> TQTQLAIDNVLASAESTIQLNELPKVVLDFITGEQTSVARSGGIFTKEDLINLKLYVRKGLSLPTRQDEVEAYLGYKKIDVAGLEPKDIKLLFDEIHNHALNWNDVEQAVLQQSLDLDIAAKNIISTGNEIINLINQMPITLRVKTLLGDITDKQLENITYESADHEVASALKDILDDMKGDINRHQTTTENVRKKVSDYRITLTGGELSSGDKVNGLEPQVKTKYDLMEKSNMRKSIKELDEKIKEKRQRIEQLKKDYDKFVGLSFTGAIGGIIAMAITGGIFGAKAENARKEKNALISEVAELESKVSSQRALQTALEALSLSFSDIGIRMVDAESALNHLDFMWLSVLNQITESQIQFAMINNALRLTSFVNKFQQVITPWQSVGDSARQLVDIFDEAIKEYKKVYG

We have unraveled structures of the soluble components and the pore assembly of the YaxAB cytolysin from Y. enterocolitica. The crystal structures show an atypical fold, comprising a head domain reminiscent of ClyA family toxins and pronounced coiled-coil and foot domains unique to the YaxAB system. In line with our finding that the isolated YaxA and YaxB head domains form spoked oligomers in solution, the YaxB head domain in isolation was sufficient for recruitment to membrane-bound YaxA. Together, our biochemical data support a role for YaxA as the initial membrane-interacting subunit of the toxin, able to bring the lytic effector YaxB to the target cell surface. Therefore, we propose that this class of toxins defines a new structural family of α-PFTs.

YaxA and PaxB crystal structures were determined using single-wavelength anomalous dispersion (SAD) on selenomethionine-derivatized proteins. Because our PaxB model could be well resolved, missing merely the N-terminal 11 residues, we will utilize these coordinates for most structural analyses throughout the manuscript. All three proteins adopt similarly elongated, α-helical folds composed of a five-helix bundle head domain and a two-helix-coiled-coil stalk, tapering to a narrow turn in the case of YaxA, while connecting to an additional α-helical domain in the case of PaxB. For alignments of the YaxA head domain, Z-scores ranged from 9.6 (soluble-monomeric ClyA, 5.5 Å RMSD; PDB code 1QOY34) to 12.2 (NheA, 3.4 Å RMSD; PDB code 4K1P26). Looking at a series of conserved and solvent-exposed hydrophobic residues of the YaxA foot domain, we suspected this moiety to be a possible membrane insertion site. Replacing individual nonpolar residues in the YaxA foot to aspartic acid (V264, L266, F268, and I272, along helix α4) resulted in 2-fold to 3-fold weaker membrane association (lanes 7–10). Strikingly, a deletion mutant of most of this domain (Δ265–284; Fig. 6c, lane 11) did not co-sediment with membranes. Reflecting their impaired membrane binding, YaxA foot domain mutants showed reduced hemolytic activity, ranging from a 10-fold decrease in potency (V264D) to undetectable activity up to 2 µM (Δ265–284). YaxA, bearing a membrane-binding domain at the tip of its coiled-coil stalk, associates with the target membrane on its own. Uncharacteristic of PFTs, YaxA’s transmembrane moiety is fully solvent exposed in its monomeric state and becomes an integral part of the pore structure upon oligomerization with YaxB. For YaxA, rearrangements in the head domain remain modest compared with the monomeric protein (RMSD of 1.1 Å across 259 Cα pairs).> MALKKAPKLFKTFFHWKLWKFSIIVFVFLVFLFLLQREVGVQDFKDEAGIEPVVGKKSHVLGLVLNAMNNIKGAKPKMQIKAPIRQTKVPGERHCLPGHYTPVELKPFLDRPLQDPNAPGASGKAFKTINLNSEEQKEKQAGEEKHCFNAFASDRISLHRDLGPDTRPPECIEQKFKRCPPLPTTSIIIVFHNEAWSTLLRTVHSVMYTSPAILLKEIILVDDASVDEYLHDKLDEYVKQFQIVKVVRQKERKGLITARLLGASVATGETLTFLDAHCECFYGWLEPLLARIAENPVAVVSPDIASIDLNTFEFSKPSPYGHSHNRGNFDWSLSFGWESLPKHENKRRKDETYPIRTPTFAGGLFSISKDYFEYIGSYDEEMEIWGGENIEMSFRVWQCGGQLEIMPCSVVGHVFRSKSPHTFPKGTQVITRNQVRLAEVWMDEYKEIFYRRNTEAAKIVKQKTFGDISKRIDLRQRLQCKNFTWYLSNVYPEAYVPDLNPLFSGYLKNIGNRMCLDVGENNHGGKPLIMYSCHGLGGNQYFEYSAHHEIRHN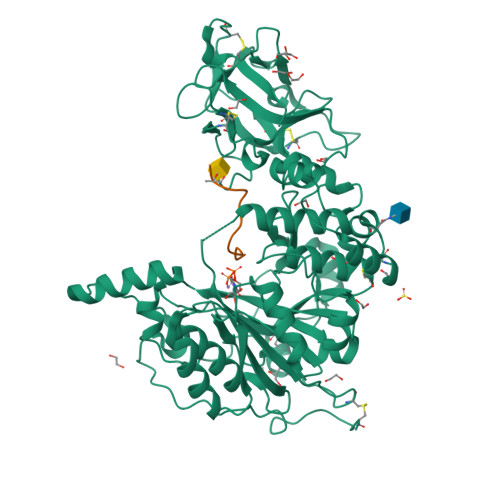IQKELCLHASKGPVQLRECTYKGQKTFAVGEEQWLHQKDQTLYNEALHMCLTGNGEHPSLASCNPSDPFQKWIFGQND;> NTPIPRRHTRSA methyl [(2S)-2-[4-({5-[4-({(2S)-2-[(3S)-3-amino-2-oxopiperidin-1-yl]-2-cyclohexylacetyl}amino)phenyl]pentyl}oxy)phenyl]-3-(quinolin-3-yl)propyl]carbamate 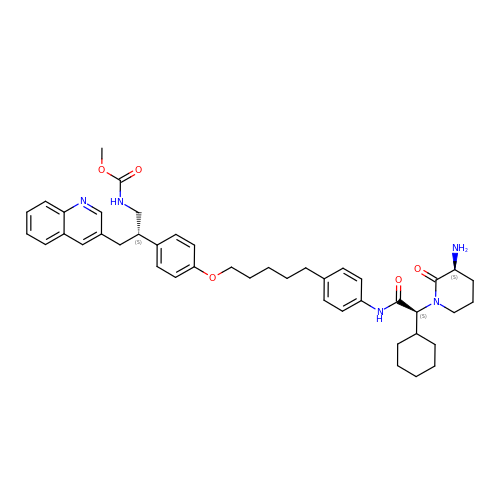| C44 H55 N5 O5 | IGRIVAWLJUPVMM-UDEWTJCRSA-N6-phenoxy-3-pyridinamine | 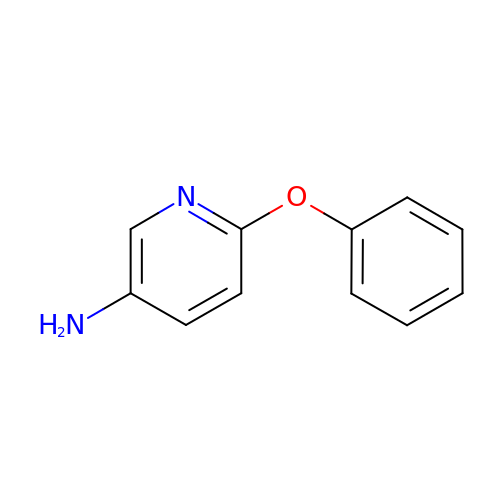C11 H10 N2 O | DETKIRMPBJPJRQ-UHFFFAOYSA-N> MSIKPCKPRDGPVTYEAEDAILTGTTVDTAQVGYTGRGYVTGFDEGSDKITFQISSATTKLYDLSIRYAAIYGDKRTNVVLNNGAVSEVFFPAGDSFTSVAAGQVLLNAGQNTIDIVNNWGWYLIDSITLTPSAPRPPHDINPNLNNPNADTNAKKLYSYLRSVYGNKIISGQQELHHAEWIRQQTGKTPALVAVDLMDYSPSRVERGTTSHAVEDAIAHHN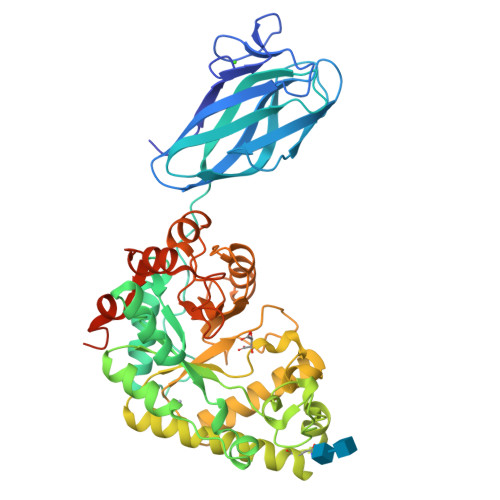AGGIVSVLWHWNAPVGLYDTEENKWWSGFYTRATDFDIAATLANPQGANYTLLIRDIDAIAVQLKRLEAAGVPVLWRPLHEAEGGWFWWGAKGPEPAKQLWDILYERLTVHHGLDNLIWVWNSILEDWYPGDDTVDILSADVYAQGNGPMSTQYNELIALGRDKKMIAAAEVGAAPLPGLLQAYQANWLWFAVWGDDFINNPSWNTVAVLNEIYNSDYVLTLDEIQGWRSGDEQKLISEEDLNSAVDHHHHHH>MGSSHHHHHHGSSAKVKKPELLIFDVNETLLDMGPLENAINESLNSEHAFSLWFRTLLHYSLTETLTGNYVDFGTIGKATLKMTMRKFGKNLSEDRLDAILGNIKKLPAHEDVKEGLKMLKEAQIKLVALSNSNGKLLNAQLQFAGLADYFDAIFSVEAVGRYK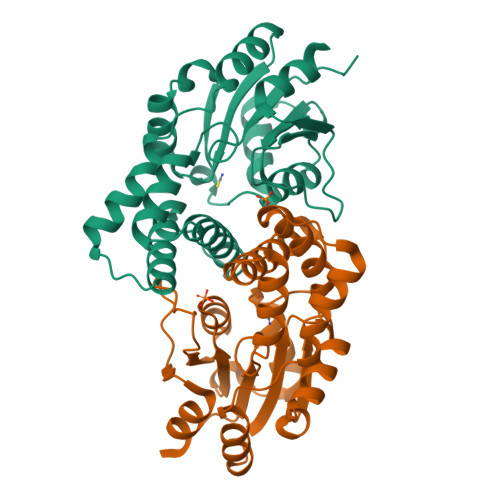PELASYRAVLETMKVPAENTMMVAAAGWDILGAKRAGLRTAFVAREGHAIYPLDGTPELEAKTVLEVARTLLKN[2x]>[2x]MRRFAAGCLALALLVLPFVLTGARAAEDESEKEIERYRQMIEDPMANPGFLNVDRGEVLWSEPRGTRNVSLE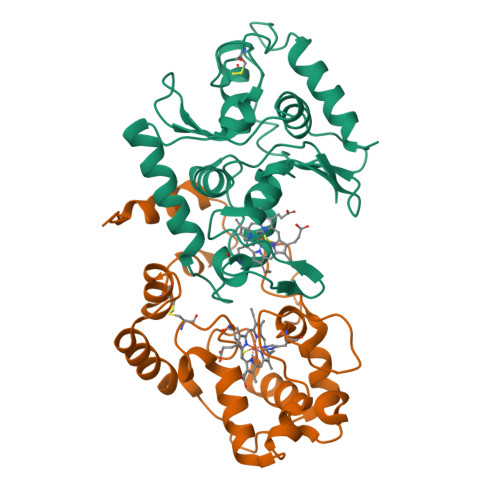TCDLGEGPGKLEGAYAHLPRYFADTGKVMDLEQRLLWCMETIQGRDTKPLVAKPFSGPGRTSDMEDLVAFIANKSDGVKIKVALATPQEKEMYAIGEALFFRRSSINDFSCSTCHGAAGKRIRLQALPQLDVPGKDAQLTMATWPTYRVSQSALRTMQHRMWDMYRQMRMPAPDYASEAVTALTLYLTKQAEGGELKVPSIKR;>MRFETLLKRAAQVGALVLLPLAAHAQEASAVDPARVDAVVKTSFTKLPEGWESRLQQDETQRICSVTRNNPSPEQAAAIMKAEEVRIKFPAGPVLGSWKDGAKVAQNGRGGQFSDPPGTVSGGNCYACHQLDPKEVSYGTLGPSLVGYGRERNFSAEDAKIAFAKVYDAQASLACSSMPRFGVNGVLTEQQIKDVVAYLFDPESPVNK[2x]> ETFDPTELPELLKLYYRRLFPYSQYYRWLNYGGVIKNYFQHREFSFTLKDDIYIRYQSFNNQSDLEKEMQKMNPYKIDIGAVYSHRPNQHNTVKLGAFQAQEKELVFDIDMTDYDDVRRCCSSADICPKCWTLMTMAIRIIDRALKEDFGFKHRLWVYSGRRGVHCWVCDESVRKLSSAVRSGIVEYLSLVKGGQDVKKKVHLSEKIHPFIRKSINIIKKYFEEYALVNQDILENKESWDKILALVPETIHDELQQSFQKSHNSLQRWEHLKKVASRYQNNIKNDKYGPWLEWEIMLQYCFPRLDINVSKGINHLLKSPFSVHPKTGRISVPIDLQKVDQFDPFTVPTISFICRELDAISTNEEEKEENEAESDVKHRTRDYKKTSLAPYVKVFEHFLENLDKSRKGELLKKSDLQKD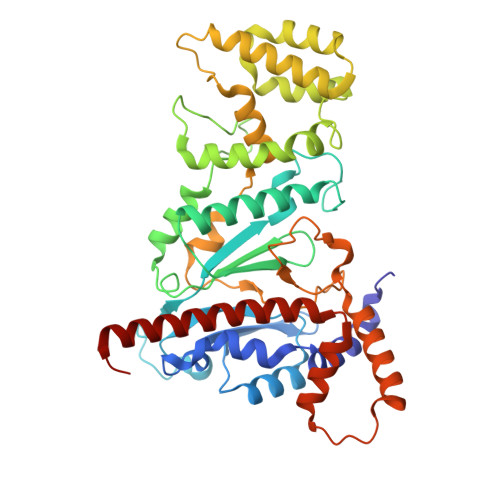F> MPKFYCDYCDTYLTHDSPSVRKTHCSGRKHKENVKDYYRNKARDIINKHNHKRRHIGKRGRKERENSSQNETLKVTCLSNKEKRHIMHVKKMNQKELAQTSIDTLKLLYDGSPGYSKVFVDANRFDIGDLVKASK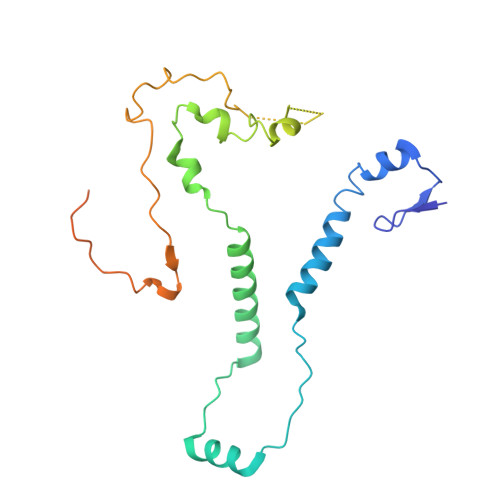LPQRANEKSAHHSFKQTSRSRDETCESNPFPRLNNPKKLEPPKILSQWSNTIPKTSIFYSVDILQTTIKESKKRMHSDGIRKPSSANGYKRRRYGN>[5x]APADNAADARPVDVSVSIFINKIYGVNTLEQTYKVDGYIVAQWTGKPRKTPGDKPLIVENTQIERWINNGLWVPALEFINVVGSPDTGNKRLMLFPDGRVIYNARFLGSFSNDMDFRLFPFDRQQFVLELEPFSYNNQQLRFSDIQVYTENIDNEEIDEWWIRGKASTHISDIRYDHLSSVQPNQNEFSRITVRIDAVRNPSYYLWSFILPLGLIIAASWSVFWLESFSERLQTSFTLML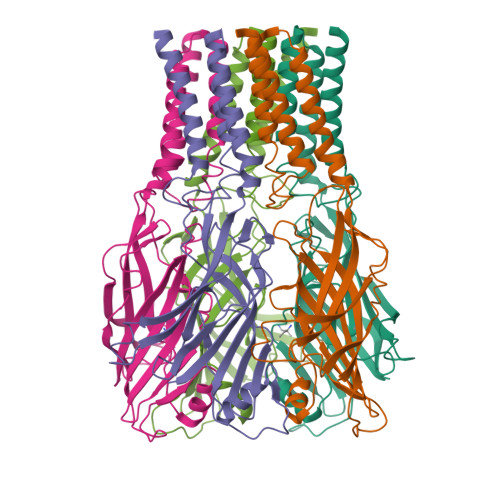TVVAYAFYTSNILPRLPYTTVIDQMIIAGYGSIFAAILLIIFAHHRQANGVEDDLLIQRCRLAFPLGFLAIGCVLVIRGITL SgvM is found in the biosynthetic gene cluster of the antibiotic viridogrisein and catalyzes methyl transfer to the C3 (i.e., β) position of α-ketoleucine (4-methyl-2-oxovalerate). The overall structure consists of a two-domain fold that assembles into homodimer in both the solution and the crystal. The N-terminal domain (I6 through H147) consists of helices that mediate dimerization, while the C-terminal domain (F149 through H338) consists of a Rossman fold. A single metal ion is located at the base of the C-terminal domain and is ligated by H244 and H296.

In order to provide further insights into the broader substrate scope and enhanced total turnover number of SgvMVAV, we determined its crystal structure in complex with SAH and 1a (2.04 Å resolution). Protein crystallography showed that although the three amino acid substitutions led to limited alterations in the overall structure, they resulted in a substantially widening of the binding pocket to accommodate larger substrates. Meanwhile, interactions between the protein, the metal ion and the bound SAH cofactor are sufficient to accommodate these dramatic changes in the active site contours with minimal perturbations to the overall scaffold. Taken together, the expanded substrate binding pocket and the retained overall enzyme scaffold allowed for a broad range of substrates to be effectively transformed, leading to a generally useful enantioselective alkylation biocatalyst. Further active site engineering showed that a single M144V mutation significantly improved enzyme activity (TTN = 1080). M144 resides in an α-helix proximal to the phenyl group of 1a. Ultimately, triple mutant SgvM F329V T331A M144V (SgvMVAV) exhibited the highest activity, furnishing excellent yield and enantiomeric ratio (e.r.) of 1a (TTN = 1,410, 93% yield and 99:1 e.r.). Compared to wt SgvM, SgvMVAV provided a 235-fold improvement in TTN, demonstrating its substantially enhanced catalytic efficiency.

> MATHDIAAQHLADGIAASGPAPDLAAAAAFLEMGDRLGVVAHLDPDRTLETAEVAAALDLPEPALVRYLDAVESAGLVIREGEGRYRACPDFDTIRHQAGYISWTMNANRPFIENARDFFTDWDKAARTHVRDYREVAVSSQWVGSHAFYPTALATIIDAAPRKVVDLGAGTCRLLIEVLGAVPGSTGVGLDFAADACRAAEQAVAQAGMTDRLTVVERTIQSVATDPGVLEGADVIHAGFVFHDMLPEEEDVCDQVLANCRESLAPGGFLAITDAVPYLRNDRERRFSAAVSYYHGEFMRRRLQSEEEWVERLRGAGFSDVRALTLAVPAGRLFLAHR> TETTSFLITKFSPDQQNLIFQGDGYTTKEKLTLTKAVKNTVGRALYSSPIHIWDRETGNVANFVTSFTFVINAPNSYNVADGFTFFIAPVDTKPQTGGGYLGVFNSAEYDKTTQTVAVEFDTFYNAAWDPSNRDRHIGIDVNSIKSVNTKSWKLQNGEEANVVIAFNAATN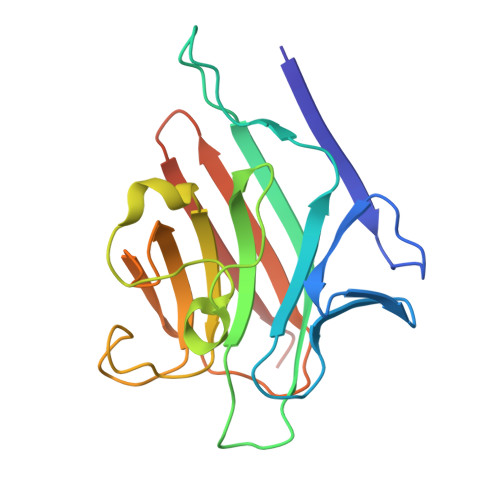VLTVSLTYPNSLEEEN>[2x]ELTPDQQTLLHFIMDSYNKQRMPQEITNKILKEEFSAEENFLILTEMATNHVQVLVEFTKKLPGFQTLDHEDQIAL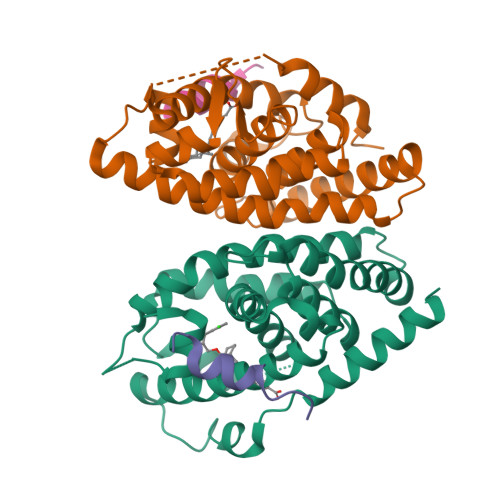LKGSAVEAMFLRSAEIFNKKLPSGHSDLLEERIRNSGISDEYITPMFSFYKSIGELKMTQEEYALLTAIVILSPDRQYIKDREAVEKLQEPLLDVLQKLCKIHQPENPQHFAELLGRLTELRTFNHHHAEMLMSWRVNDHKFTPLLEEIWDVQ;>SANEDMPVERILEAELAVEPKTETYVEANMGLNPSSPNDPVTNICQAADKQLFTLVEWAKRIPHFSELPLDDQVILLRAGWNELLIASFSHRSIAVKDGILLATGLHVHRNSAHSAGVGAIFDRVLTELVSKMRDMQMDKTELGCLRAIVLFNPDSKGLSNPAEVEALREKVYASLEAYCKHKYPEQPGRFAKLLLRLPALRSIGLKCLEHLFFFKLIGDTPIDTFLMEMLEAPHQMT[2x];>ERHKILHRLLQEGSPS[4x]OXYTETRACYCLINE 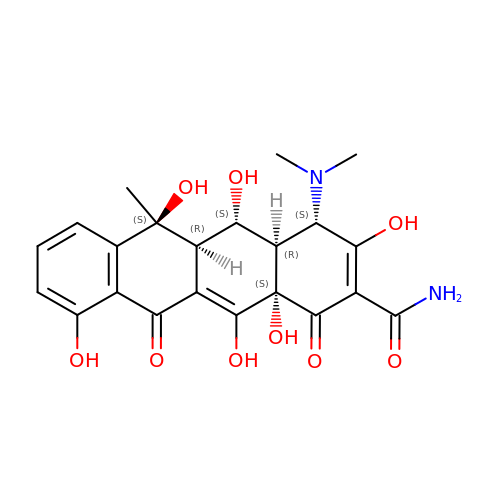| C22 H24 N2 O9 | IWVCMVBTMGNXQD-PXOLEDIWSA-N> GSQRWRSDGRCGPNYPAPDANPGECNPHAVDHCCSEWGWCGRETSHCTCSSCVDYSAGSSGTCPRIVSKSEWGSRATNYNVFLSLPVPKVVIHHSAGATCSTQSSCSLQVRNIQNYHMDGR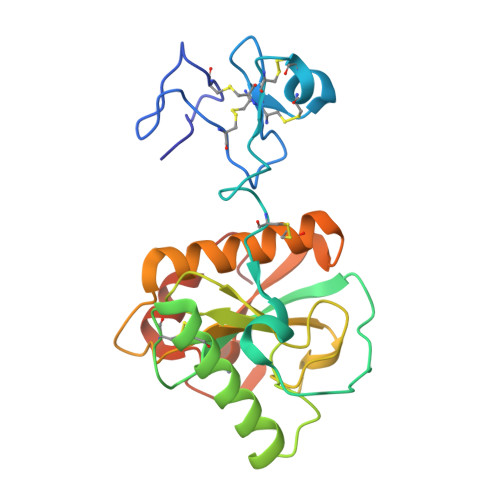GYSDIGYNFLVGNDGNVYEGRGWDRRGAHALNVNTESIGICFMGDFTSQKPTASAIAAAKSLISCGVSLGKIRSGYSLYGHRDVGSTACPGNLLYDDIKSWGRYVGAAAHHHHHH>[3x]MSSERTFIAVKPDGVQRGLVGEIIARFERKGYKLVALKILQPTTEQAQGHYKDLCSKPFFPALVKYFSSGPIVCMVWEGKNVVKS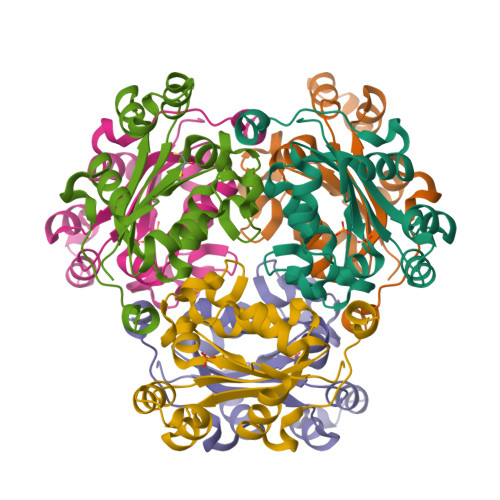GRVLLGATNPADSQPGTIRGDFAVDVGRNVCHGSDSVESAEREIAFWFKADEIASWTSHSVSQIYE> GDPYWAYSGAYGPEHWVTSSVSCGGRHQSPIDILDQYARVGEEYQELQLDGFDNESSNKTWMKNTGKTVAILLKDDYFVSGAGLPGRFKAEKVEFHWGHSNGSAGSEHSINGRRFPVEMQIFFYNPDDFDSFQTAI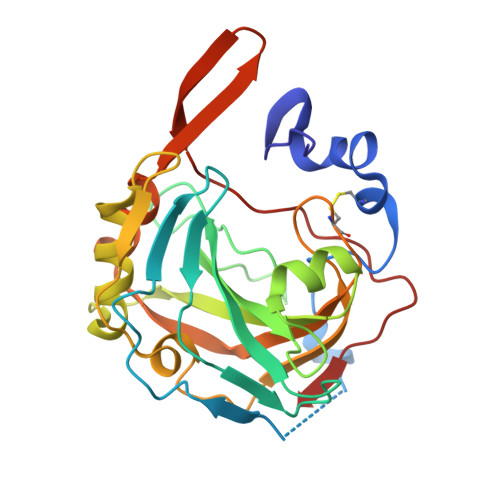SENRIIGAMAIFFQVSPRDNSALDPIIHGLKGVVHHEKETFLDPFVLRDLLPASLGSYYRYTGSLTTPPCSEIVEWIVFRRPVPISYHQLEAFYSIFTTEQQDHVKSVEYLRNNFRPQQRLHDRVVSKS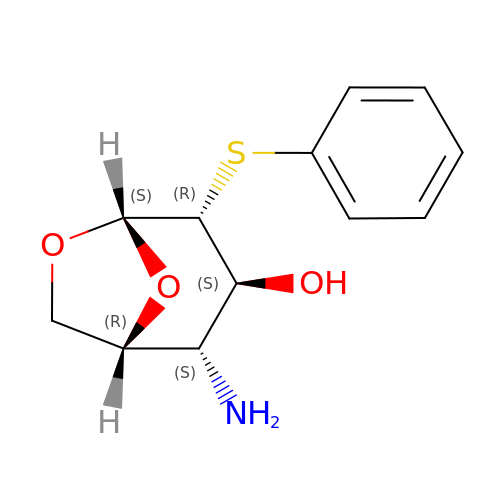(1~{R},2~{S},3~{S},4~{R},5~{S})-2-azanyl-4-phenylsulfanyl-6,8-dioxabicyclo[3.2.1]octan-3-ol | C12 H15 N O3 S | OFCUYBHPAYPQJR-MJDLHHQISA-N>MEQNKCALVTGSSRGVGKAAAIRLAENGYNIVINYARSKKAALETAEEIEKLGVKVLVVKANVGQPAKIKEMFQQIDETFGRLDVFVNNAASGVLRPVMELEETHWDWTMNINAKALLFCAQEAAKLMEKNGGGHIVSISSLGSIRYLENYTTVGVSKAALEALTRYLAVELSPKQIIVNAVSGGAIDTDALKHFPNREDLLEDARQNTPAGRMVEIKDMVDTVEFLVSSKADMIRGQTIIVDGGRSLLVL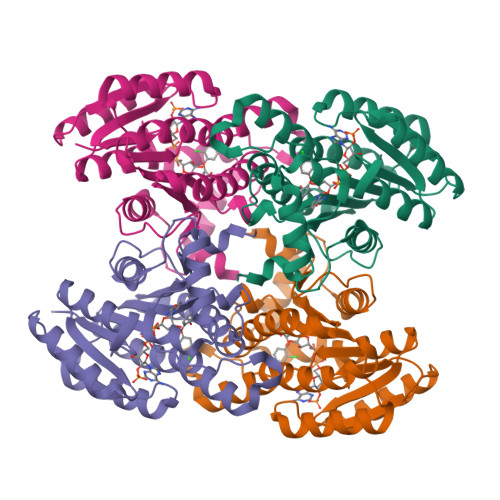EHHHHHH[4x]> ASWSHPQFEKGAELPVQRWWHKGALYRIGDLQAFVGRDAGGIAGLKSHLEYLSTLKVKGLVLGPIHKNQKDEINETDLKQINPTLGSQEDFKDLLQSAKKKSIHIILDLTPNYQGQNAWFLPAQADIVATKMKEALSSWLQDGVD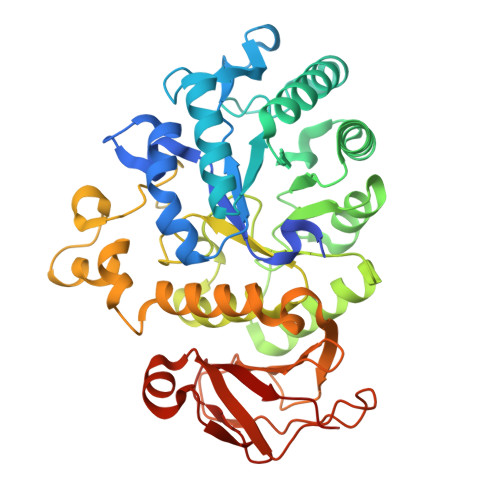GFQFRDVGKLMNAPLYLAEWQNITKNLSEDRLLIAGTESSDLQQIVNILESTSDLLLTSSYLSNSTFTGERTESLVTRFLNATGSQWCSWSVSQAGLLADFIPDHLLRLYQLLLFTLPGTPVFSYGDELGLQGALPGQPAKAPLMPWNESSIFHIPRPVSLNMTVKGQNEDPGSLLTQFRRLSDLRGKERSLLHGDFHALSSSPDLFSYIRHWDQNERYLVVLNFRDSGRSARLGASNLPAGISLPASAKLLLSTDSARQSREEDTSLKLENLSLNPYEGLLLQFPFVA> MTTLLNPYFGEFGGMYVPQILMPALNQLEEAFVRAQKDPEFQAQFADLLKNYAGRPTALTKCQNITAGTRTTLYLKREDLLHGGAHTTNQVLGQALLAKRMGKSEIIAETGAGQHGVASALASALLGLKCRIYMGAKDVERQSPNVFRMRLM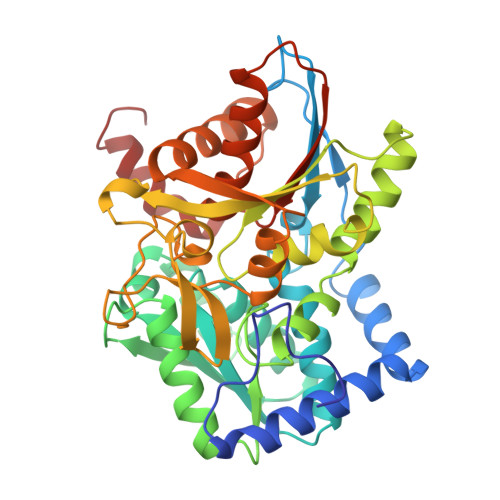GAEVIPVHSGSATLKDACNEALRDWSGSYETAHYMLGTAAGPHPYPTIVREFQRMIGEETKAQILDKEGRLPDAVIACVGGGSNAIGMFADFINDTSVGLIGVEPGGHGIETGEHGAPLKHGRVGIYFGMKAPMMQTADGQIEESYSISAGLDFPSVGPQHAYLNSIGRADYVSITDDEALEAFKTLCRHEGIIPALESSHALAHALKMMREQPEKEQLLVVNLSGRGDKDIFTVHDILKARGEI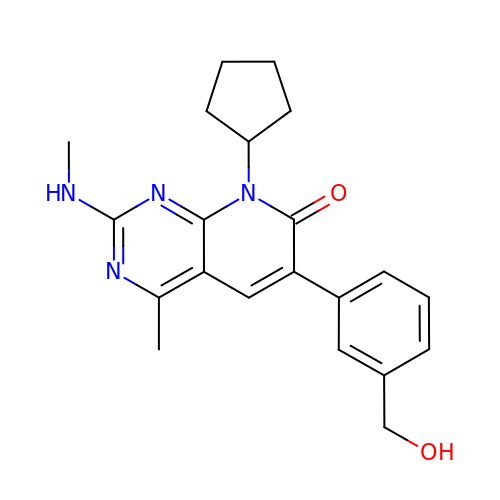8-cyclopentyl-6-[3-(hydroxymethyl)phenyl]-4-methyl-2-(methylamino)pyrido[2,3-d]pyrimidin-7(8H)-one | C21 H24 N4 O2 | LASGWNJRSNLLFV-UHFFFAOYSA-N>[2x]MSKSPYVDPHKSGHEIWEEFSMSFTPAVKEVVEFAKRIPGFRDLSQHDQVNLLKAGTFEVLMVRFASLFDAKERTVTFLSGKKYSVDDLHSMGAGDLLNS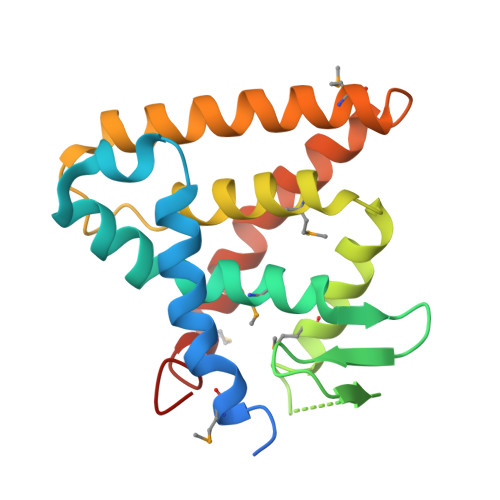MFEFSEKLNALQLSDEEMSLFTAVVLVSADRSGIENVNSVEALQETLIRALRTLIMKNHPNEASIFTKLLLKLPDLRSLNNMHSEELLAFKVHP> MVGSLNCIVAVSQNMGIGKNGDLPWPPLRNEFRYFSRMTTTSSVEGKQNLVIMGKKTWFSIPEKFRPLKGRINLVLSRELKEPPQGAHFLSRSLDDALKLTEQPELANKVDMV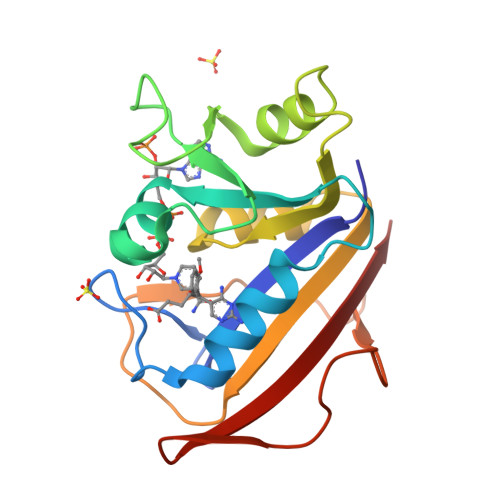WIVGGSSVYKEAMNHPGHLKLFVTRIMQDFESDTFFPEIDLEKYKLLPEYPGVLSDVQEEKGIKYKFEVYEKND> NL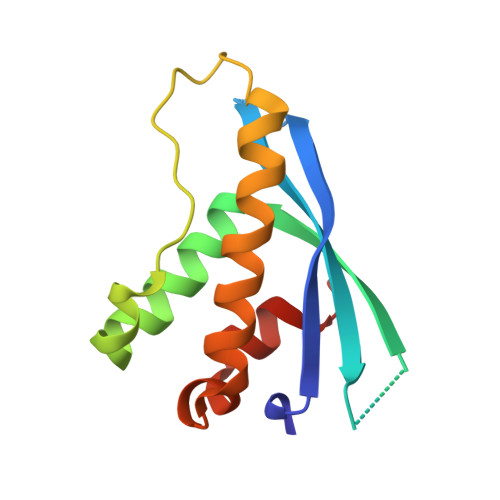GTWRAVVSTAEASEENGEQMACYFVAVSLSEEDDCKNNHWTVSRKLIEFQALHRKLTECFPSLKKVQLPSLSKLPFKSIDQKFLDKSKNQLNAFLQKVLTDERMCQSEALYAFLSPSLE> CAAAGAAAAG;> CTTTTCTTTG

With this in mind we describe reduced-charge oligonucleotides containing artificial LNA-amide linkages with improved gymnotic cell uptake, RNA affinity, stability and potency. We solved several X-ray structures to determine the effects of LNA and amide modifications on duplex structure and conformation. These are the first crystal structures of DNA:RNA hybrids that contain amide linkages. The sequence of the modified DNA:RNA hybrid duplexes was based on the corresponding unmodified version (d-CTTTTCTTTG/rCAAAGAAAAG)51 (the location of the amide is underlined).

The unmodified DNA:RNA duplex was also studied. The hybrids with amide and LNA-amide backbones are structurally very similar to the unmodified duplex (all-atom RMSD 0.4 Å) as shown by their superimposition. All structures adopt the A-conformation with sugar puckers clustering around C3′-endo. As expected, all duplexes are stabilised by canonical Watson–Crick base pairs, indicating that the thermodynamic improvements due to the LNA-amide backbones are not due to unusual changes in hydrogen bonding interactions.>[2x]MLEKVEEWIKARGLTWRLLIMQKPTRTVAEAAALLGVSESEIVKTLIVLDNAGGVYAVVIPGDKRLNINSMKELAGKPVRLARANEVVELTGYPVGGVPPVAL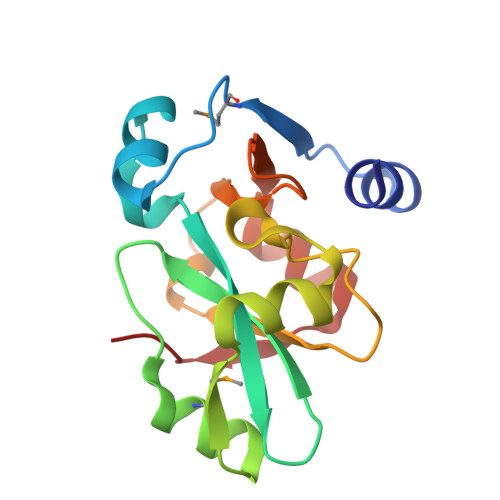PPNIVLVVDRILLSRKKVYGGGGRENALLEFSPRELVEATGAVVADVSE>[2x]MVSRYVPDMGDLIWVDFDPTKGSAQAGHRPAVVLSPFMYNN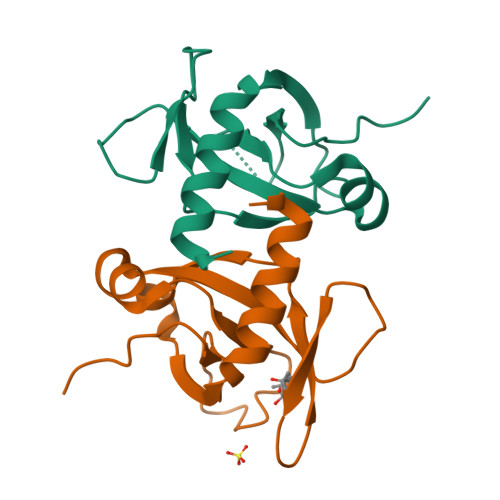KTGMCLCVPCTTQSKGYPFEVVLSGQERDGVALADQVKSIAWRARGATKKGTVAPEELQLIKAKINVLIGLSHHHHHH> GAMGSNLSVEAEVDLLSYCAREWKGETPRNKLMRKAYEELFWRHH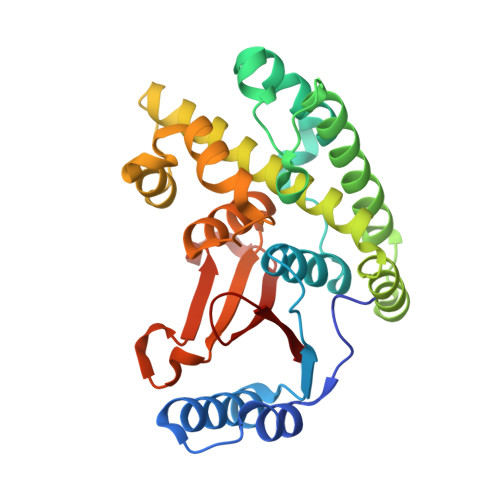IKCVRQVRRDNYDALRSVLFQIFSQGISFPSWMKEKDIVKLPEKLLFSQGCNWIQQYSFGPEKYTGSNVFGKLRKYVELLKTQWTEFNGIRDYHKRGSMCNTLFSDAILEYKLYEALKFIMLYQVTEVYEQMKTKKVIPSLFRLLFSRETSSDPLSFMMNHLNSVGDTCGLEQIDMFILGYSLEVKIKVFRLFKFNSRDFEVCYPEEPLRDWPEISLLTENDRHYHIPVF>[2x]SLLENAEEEKERQIASILSWEIDIIYKILLDSDLGSSLPLSQADFGLWFNHKGRHYFSGIAEVGHISRLIQDFDGIFNQTMRNTRNLNNRSLRVKFLLQIRNTVS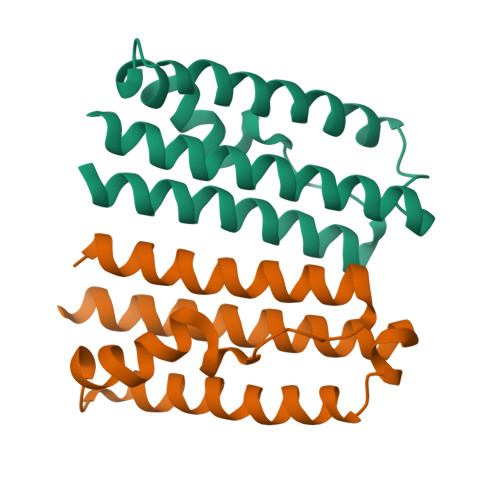QIITLLRELFEEVSRHEVGMD In this work, we exhaustively probe the ability of all 36 immobile HJ sequences to form DNA crystals in two different designed systems. Three separate self-assembling DNA crystal systems are described in this report: the “4 × 5” and “4 × 6” designs (collectively referred to as the 4 × N systems), and a third construct with a “scrambled” sequence variant of the 4 × 6 lattices. Self-assembly was mediated by three constituent oligonucleotides: (S1) containing four sequence repeats of either 5 or 6 bases; (S2) composed of 21 bases containing complementary regions to both (S1); and (S3) which forms the second junction crossover. The HJ serves as the fundamental component at the core of each unit, and the ultimate assembly of the full lattice is facilitated by the complementary 2-base sticky ends that tail each duplex.

Each asymmetric unit could be defined as either a HJ containing 10 and 11 bp on each arm, or as a 21-bp linear duplex. In parallel, we employed the previously reported J1 4 × 6 system (3.05 Å), with P32 symmetry. Seventeen of the 36 junctions successfully crystallized, a 47% success rate. Unlike the 4 × 5 motif, nearly all of the 4 × 6 junction sequences had a strong preference for crystallization in buffers containing ≥2.0 M salts (e.g., LiCl, Li2SO4, KCl, and NaCl), with the majority preferring slightly basic pH conditions in cacodylic acid. The average cell constants for the P32 crystals were a = b = 68.29 Å c = 55.68 Å. However, in the majority of the crystal structures reported here, the cacodylate anion indeed fits best into the electron density map of our X-ray structures, due to the presence of sodium cacodylate in the crystallization solution.

> GAGCAGACTTGACGAGACTCA;> TCGTCA;> TCTGAGTC;> AGTCTGC> MGTYAVAFRLERGLVFAADTRTNAGVDNIAQYKKLQLWRQPGERVFVLLSAGNLAATQA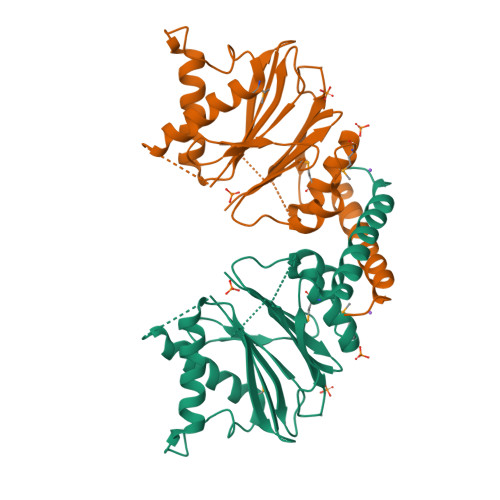VVSLINEHLSQETDDEVTTLFTAPNMYRAARVVGDAVREARSIDGAALEASKLGFNTNFIFGGQIKGERPRLFQIYPEGNFIEATDDTPFFQIGEHKYGKPILDRVARSDMRLGEAAKLMLLSFDSTLRSNLSVGMPIDLVIYERDTFDVTREKRISADDEYFRNLSNAWSDALRQAFSKIEEFDV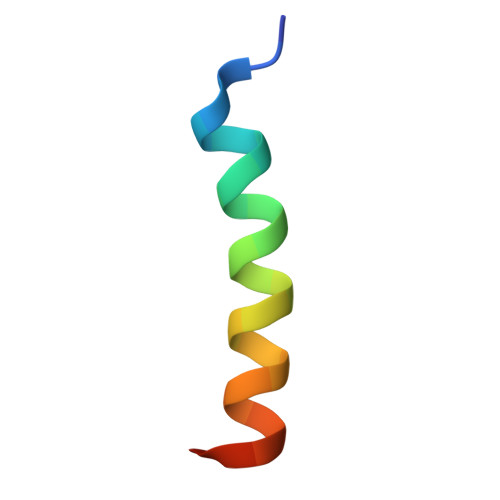> ALPPEMVVARELRRIGDEFNRLYCEA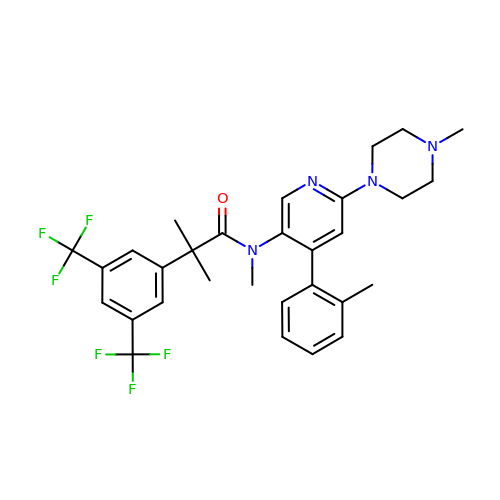2-[3,5-bis(trifluoromethyl)phenyl]-~{N},2-dimethyl-~{N}-[4-(2-methylphenyl)-6-(4-methylpiperazin-1-yl)pyridin-3-yl]propanamide | C30 H32 F6 N4 O | WAXQNWCZJDTGBU-UHFFFAOYSA-N> GGGCUGCACUUCGGUGCUGCCC

Here, we report the crystal structure of an RNA that contains a CUG repeat and a UUCG sequence. The RNA was designed to form a hairpin with an isolated CUG repeat [Fig. 1(a)] to provide a platform for analyzing compounds designed to target the CUG repeat sequence. Instead, the RNA crystallized into a duplex in which the two CUG repeats are related by twofold symmetry and form a U–U mismatch flanked by C–G pairs.

For the purposes of discussion, we give one strand in the duplex the numbering 1–22 and the other 1′–22′. The RNA adopts an A-form geometry for all nucleotides except the UUCG sequence regions, which are involved in crystal contacts [Figs. 1(d) and 2(a)]. All ribose sugar puckers are C3′-endo, with the exception of U11 and U11′, which are C2′-endo. The UUCG region forms an unusual structure, with two U–C base pairs that are cross-strand stacked [Fig. 2(b)]. The U–C base pairs form a hydrogen bond between the uracil O2 and the cytosine N3 amino group. An additional inter-strand hydrogen bond is formed between the uracil N3 and the uracil ribose O2′. This conformation is significantly different from previous structures of the same sequence, which lacked cross-strand stacking [Fig. 2(c)]. The cross-strand stacked U–C base pairs are flanked by U–G wobble pairs. The CUG repeat structure is composed of a Watson–Crick C–G pair, a noncanonical U–U pair with two hydrogen bonds and a Watson–Crick G–C pair. To our knowledge, the dimerized UUCG structure reported here is a very rare example of a pyrimidine-only interaction with extensive cross-strand stacking.> MASMTGGQQMGRGSEFMIASVRGEVLEVALDHVVIEAAGVGYRVNATPATLATLRQGTEARLITAMIVREDSMTLYG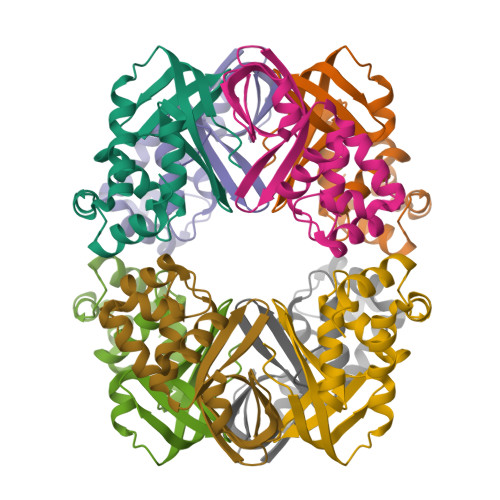FPDGETRDLFLTLLSVSGVGPRLAMAALAVHDAPALRQVLADGNVAALTRVPGIGKRGAERMVLELRDKVGVAATGGALSTNGHAVRSPVVEALVGLGFAAKQAEEATDTVLAANHDATTSSALRSALSLLGKAR> SDKQKAINYLMQFAHKVSGKYRGVAKLEGNTKAKVLQVLATFAYADYCRSAATPGARCRDCHGTGRAVDIAKTKLWGRVVEKECGRCKGVGYSR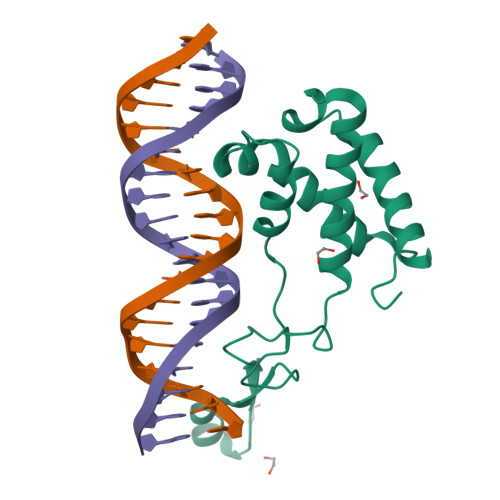MPASAAYRAVTMLIPNLTQPTWSRTVKPLYDALVVQCHKEESIADNILNAVTR6-(2,6-DICHLOROPHENYL)-2-{[3-(HYDROXYMETHYL)PHENYL]AMINO}-8-METHYLPYRIDO[2,3-D]PYRIMIDIN-7(8H)-ONE 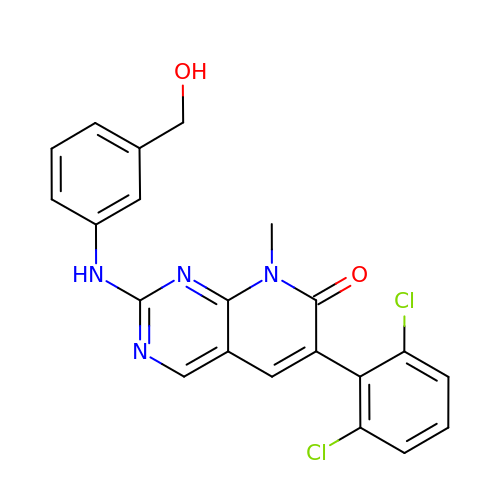| C21 H16 Cl2 N4 O2 | ZIQFYVPVJZEOFS-UHFFFAOYSA-N> MASMQELYLLGVVPSRRFEAVVNS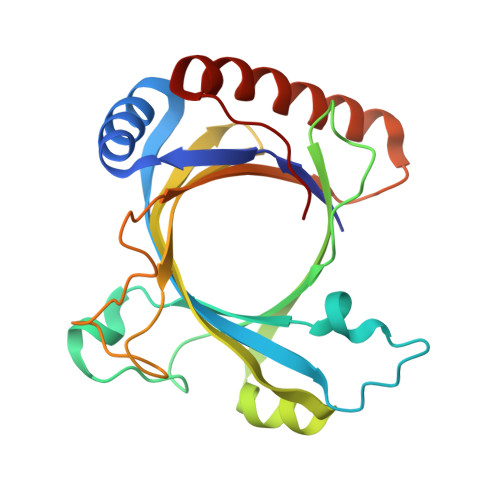LSKTLDGPKTILEFWVVYRPKDVPPNLPRQPDSWLRLCSNIESHDETDTEWSKNTQWSMYLEGNSEPKREDKCGIRPVNRAKLTNGSVTEFVEKMGYEFSHEYIIQGLEYFFFDTTVRIYQTLIPSQQRSIKPPFHPMNEEQPWILHVYTHVADASNQVAMAKAEANLTKVKTLLSAFCDLKNVRL>TPEMPVLENRAAQGDITAPGGARRLTGDQTAALRDSLSDKPAKNIILLIGDGMGDSEITAARNYAEGAGGFFKGIDALPLTGQYTHYALNKKTGKPDYVTDSAASATAWSTGVKTYNGALGVDIHEKDHPTILEMAKAAGLATGNVSTAELQDATPAALVAHVTSRKCYGPSATSEKCPGNALEKGGKGSITEQLLNARADVTLGGGAKTFAETATAGEWQGKTLREQAQARGYQLVSDAASLNSVTEANQQKPLLGLFADGNMPVRWLGPKATYHGNIDKPAVTCTPNPQRNDSVPTLAQMTDKAIELLSKNEKGFFLQVEGASIDKQDHAANPCGQIGETVDLDEAVQRALEFAKKEGNTLVIVTADHAHASQIVAPDTKAPGLTQALNTKDGAVMVMSYGNSEEDSQEHTGSQ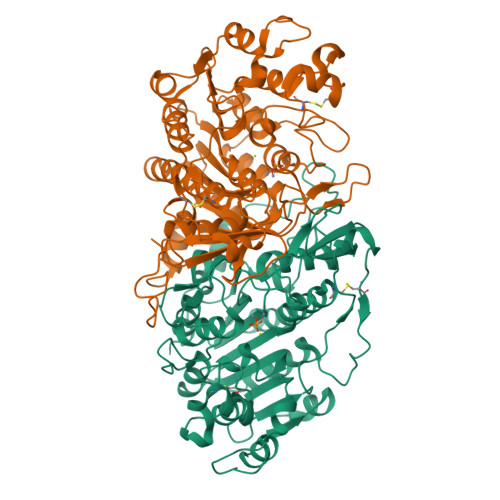LRIAAYGPHAANVVGLTDQTDLFYTMKAALGLK[4x]> GGSKMEYEWKPDEQGLQQILQLLKESQSPDTTIQRTVQQKLEQLNQYPDFNNYLIFVLTKLKSEDEPTRSLSGLILKNNVKAHFQNFPNGVTDFIKSECLNNIGDSSPLIRATVGILITTIASKGELQNWPDLLPKLCSLLDSEDYNTCEGAFGALQKICEDSAEILDSDVLDRPLNIMIPKFLQFFKHSSPKIRSHAVACVNQFIISRTQALMLHIDSFIENLFALAGDEEPEVRKNVCRALVMLLEVRMDRLLPHMHNIVEYMLQRTQDQDENVALEACEFWLTLAEQPICKDVLVRHLPKLIPVLVNGMKYSDIDIILLKGDVEEDETIPDSEQDIRPRFHRSRTVAQQHDEDGIEEEDDDDDEIDDDDTISDWNLRKCSAAALDVLANVYRDELLPHILPLLKELLFHHEWVVKESGILVLGAIAEGCMQGMIPYLPELIPHLIQCLSDKKALVRSITCWTLSRYAHWVVSQPPDTYLKPLMTELLKRILDSNKRVQEAACSAFATLEEEACTELVPYLAYILDTLVFAFSKYQHKNLLILYDAIGTLADSVGHHLNKPEYIQMLMPPLIQKWNMLKDEDKDLFPLLECLSSVATALQSGFLPYCEPVYQRCVNLVQKTLAQAMLNNAQPDQYEAPDKDFMIVALDLLSGLAEGLGGNIEQLVARSNILTLMYQCMQDKMPEVRQSSFALLGDLTKACFQHVKPCIADFMPILGTNLNPEFISVCNNATWAIGEISIQMGIEMQPYIPMVLHQLVEIINRPNTPKTLLENTAITIGRLGYVCPQEVAPMLQQFIRPWCTSLRNIRDNEEKDSAFRGICTMISVNPSGVIQDFIFFCDAVAS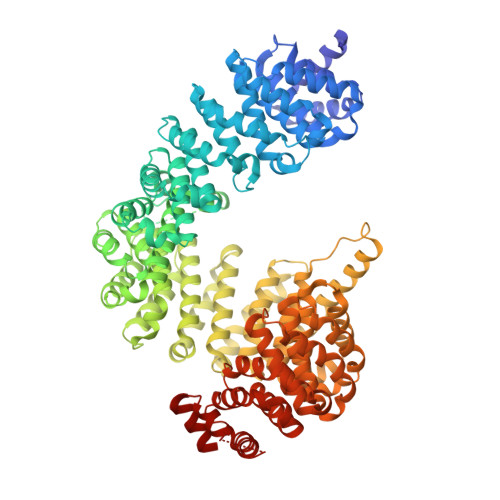WINPKDDLRDMFCKILHGFKNQVGDENWRRFSDQFPLPLKERLAAFYGV>MEHHHHHHATNLRGVMAALLTPFDQQQALDKASLRRLVQFNIQQGIDGLYVGGSTGEAFVQSLSEREQVLEIVAEEAKGKIKLIAHVGCVSTAESQQLAASAKRYGFDAVSAVTPFYYPFSFEEHCDHYRAIIDSADGLPMVVYNIPALSGVKLTLDQINTLVTLPGVGALKQTSGDLYQMEQIRREHPDLVLYNGYDNIFASGLLAGADGGIGSTYNIMGWRYQGIVKALKEGDIQTAQKLQTECNKVIDLLIKTGVFRGLKTVLHY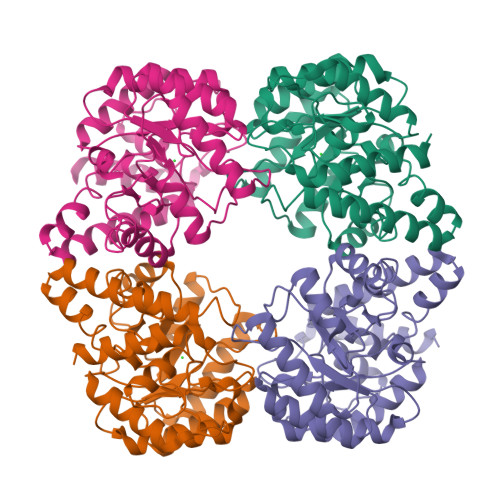MDVVSVPLCRKPFGPVDEKYLPELKALAQQLMQERG[4x]> GSHMDSLRPKLSEEQQRIIAILLDAHHKTYDPTYSDFCQFRPPVRVNDGGGSVTLELSQLSMLPHLADLVSYSIQKVIGFAKMIPGFRDLTSEDQIVLLKSSAIEVIMLRSNESFTMDDMSWTCGNQDYKYRVSDVTKAGFSLELIEPLIKFQVGLKKLNLHEEEHVLLMAICIVSPDRPGVQDAALIEAIQDRLSNTLQTYIRCRHPPPGSHLLYAKMIQKLAD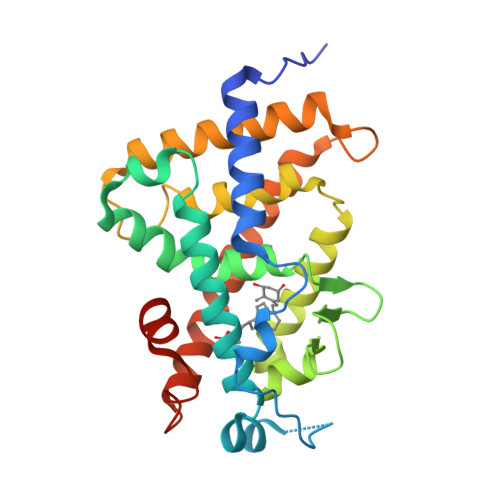LRSLNEEFSKQYRCLSFQPECSMKLTPLVLEVFGNEIS>[4x]MGACPPKAKGPWAQLQKLLISWPVGEQDWEQYRDRVNMLQQERIRDSPLLQAAKENDLRLLKILLLNQSCDFQQRGAVGETALHVAALYDNLEAATLLMEAAPELAKEPALCEPFVGQTALHIAVMNQNLNLVRALLARGASVSARATGAAFRRSPHNLIYYGEHPLSFAACVGSEEIVRLLIEHGADIRAQDSLGNTVLHILILQPNKTFACQMYNLLLSYDEHSDHLQSLELVPNHQGLTPFKLAGVEGNTVMFQHLMQKRKHVQWTCGPLTSTLYDLTEIDSWGEELSFLELVVSSKKREARQILEQTPVKELVSFKWKKYGRPYFCVLASLYILYMICFTTCCIYRPLKLRDDNRTDPRDITILQQKLLQEAYVTHQDNIRLVGELVTVTGAVIILLLEIPDIFR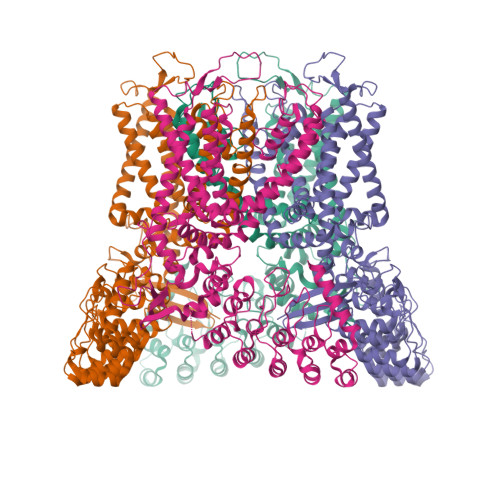VGASRYFGQTILGGPFHVIIITYASLVLLTMVMRLTNMNGEVVPLSFALVLGWCSVMYFARGFQMLGPFTIMIQKMIFGDLMRFCWLMAVVILGFASAFHITFQTEDPNNLGEFSDYPTALFSTFELFLTIIDGPANYSVDLPFMYCITYAAFAIIATLLMLNLFIAMMGDTHWRVAQERDELWRAQVVATTVMLERKMPRFLWPRSGICGYEYGLGDRWFLRVENHHDQNPLRVLRYVEAFKCSDKEDGQEQLSEKRPSTVESGMLSRASVAFQTPSLSRTTSQSSNSHRGWEILRRNDLGHLNLGLDLGEGDGEEVYHFTETSQVAPA> ALEEAPWPPPEGAFVGFVLSRKEPMWADLLALAAARGGRVHRAPEPYKALRDLKEARGLLAKDLSVLALREGLGLPPGDDPMLLAYLLDPSNTTPEGVARRYGGEWTEEAGERAALSERLFANLWGRLEGEERLLWLYREVERPLSAVLAHMEATGVRLDVAYLRAMSLEVAEEIARLEAEVFRLAGHPFNLNSRDQLERVLFDELGLPAIGKTEKTGKRSTRAAVLEALREAHPIVEKILQYRELTKLKSTYIDPLPDLIHPRTGRLHTRFNQTATATGRLSSSDPNLQNIPVRTPLGQRIRRAFIAEEGWLLVALDYSQIELRVLAHLSGDENLIRVFQEGRDFHTETASWMFGVPREAVDPLMRRAAKTINFGVLYGMSAHRLSQELAIPYEEAQAFIERYFQSFPKVRAWIEKTLEEGRRRGYVETLFGRRRYVPDLEARVKS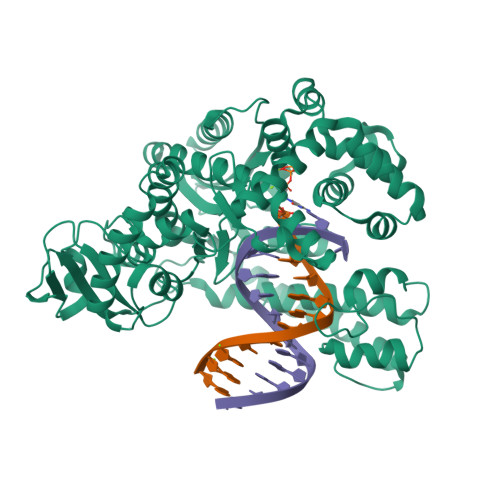VREAAERKAFNMPVQGTAADLMKLAMVKLFPRLEEMGARMLLQVHDELVLEAPKERAEAVARLAKEVMEGVYPLAVPLEVEVGIGEDWLSAKE> SGIVPQLQNIVSTVNLGCKLDLKTIALRARNAEYNPKRFAAVIMRIREPRTTALIFSSGKMVCTGAKSEEQSR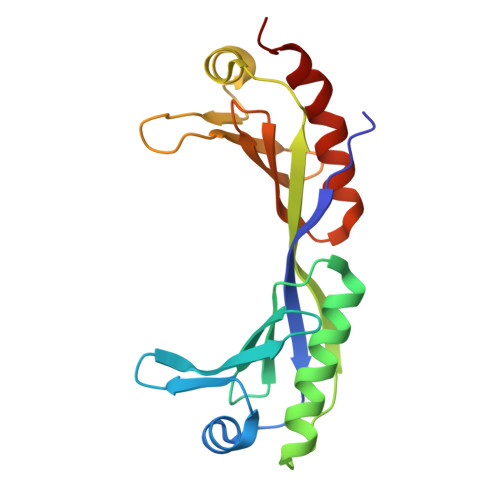LAARKYARVVQKLGFPAKFLDFKIQNMVGSCDVKFPIRLEGLVLTHQQFSSYEPELFPGLIYRMIKPRIVLLIFVSGKVVLTGAKVRAEIYEAFENIYPILKGFRKTT>[2x]MLDAYIYAGLRTPFGRHAGALSTVRPDDLAGLLLARLAETSGFAVDDLEDVILGCTNQAGEDSRNLARNALLAAGLPARLPGQTVNRLCASGLSAVIDAARAISCGEGRLYLAGGAESMSRAPFVMGKAESAFSRTLEVFDSTIGARFANPRLVERYGNDSMPETGDNVARAFGIAREDADRFAASSQARYQAALEEGFFLGEILPVEVRAGRKGETRLVERDEHPRPQADLAALARLPAL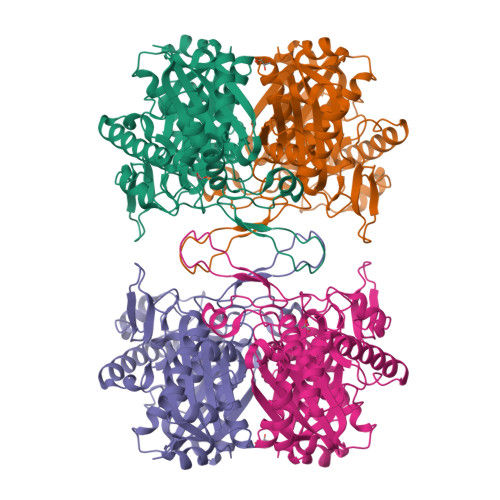FAGGVVTAGNASGINDGAAVVLLGDRAIGEREGIRPLARILASASVGVEPRLMGIGPQQAILRALQRAGIDLDEVGLIEINEAFAPQVLACLKLLGLDYEDPRVNPHGGAIALGHPLGASGARLVLTAARGLQRIERRYAVVSLCVGLGQGVAMVIERCRLEHHHHHH>[2x]MAESADELLALLTSVRQGMTAGEVAAHFGWPLEKARNALEQ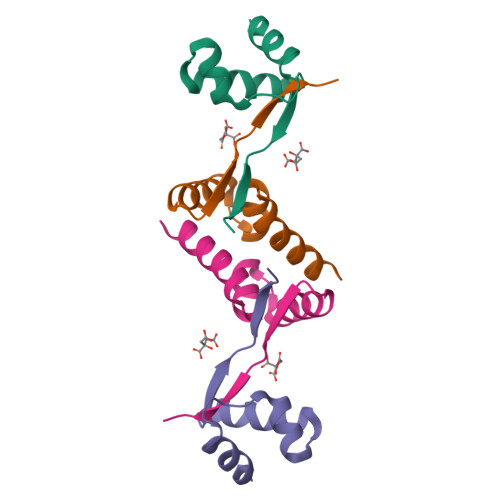LFSAGTLRKRSSRYRLKPHLEHHHHHH Glucosamine-6-phosphate N-acetyltransferase 1 (GNA1) produces GlcNAc-6-phosphate from GlcN-6-phosphate and acetyl coenzyme A. Early mercury-labelling experiments implicated a conserved cysteine in the reaction mechanism, whereas recent structural data appear to support a mechanism in which this cysteine plays no role. GlcN-6P is then acetylated by the enzyme glucos­amine-6-phosphate N-acetyltransferase 1 (GNA1), followed by conversion to GlcN-1P by a phosphomutase (AGM1) and finally generation of UDP-GlcNAc by the action of a pyrophosphorylase. GNA1 is a member of the Gcn5-related N-acetyltransferase (GNAT) superfamily. Here, two crystal structures of Caenorhabditis elegans GNA1 are reported, revealing an unusual covalent complex between this cysteine and the coenzyme A product.

Strikingly, however, we observed that a stable covalent complex between CoA and the enzyme can be formed, involving a disulfide bond to the conserved cysteine, as revealed by the 1.55 Å resolution crystal structure. This modification inactivates the enzyme, which can be reversed with reducing agents. In the structure of the covalent CoA complex the cysteine has shifted (maximum atom shifts of 4.0 Å for the side chain and 2.0 Å for the backbone) and rotated (124° around χ1) from its buried position into an exposed position on the wall of the active site, positioning it at a distance of 2.0 Å from the CoA thiol. Further significant conformational changes have also taken place. Tyr149, the residue that is thought to stabilize the negative charge developed on the CoA thiol in the proposed reaction mechanism, has rotated away from the active site (130° around χ1). A control protein sample taken immediately after purification had a mean mass of 18 876 ± 36 Da, whereas the protein from the dissolved crystals showed a mean mass of 19 654 ± 21 Da. The calculated difference mass of 777 Da is compatible with the theoretical mass of CoA (768 Da). Thus, mass spectrometry shows the presence of the enzyme–CoA adduct, in agreement with the crystallographic data.

>MSHIFDASVLAPHIPSNLPDNFKVRPLAKDDFSKGYVDLLSQLTSVGNLDQEAFEKRFEAMRTSVPNYHIVVIEDSNSQKVVASASLVVEMKFIHGAGSRGRVEDVVVDTEMRRQKLGAVLLKTLVSLGKSLGVYKISLECVPELLPFYSQFGFQDDCNFMTQRF[2x]6-[2-methyl-3-oxidanyl-5-(phosphonooxymethyl)pyridin-4-yl]-4-oxidanylidene-hexanoic acid | C13 H18 N O8 P | 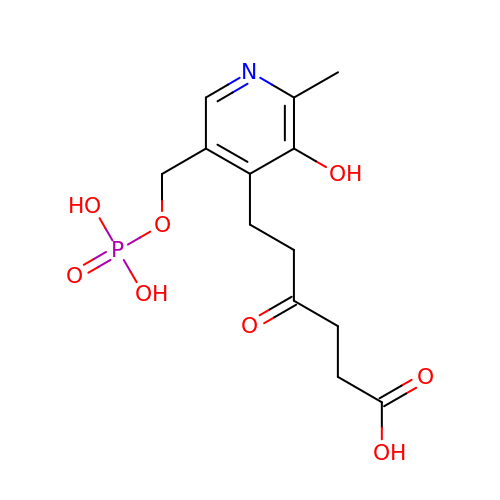QNTFLQLZXLXUGE-UHFFFAOYSA-N5-(3,5-dimethyl-1,2-oxazol-4-yl)-1-[2-(morpholin-4-yl)ethyl]-2-[2-(4-propoxyphenyl)ethyl]-1H-benzimidazole | C29 H36 N4 O3 | 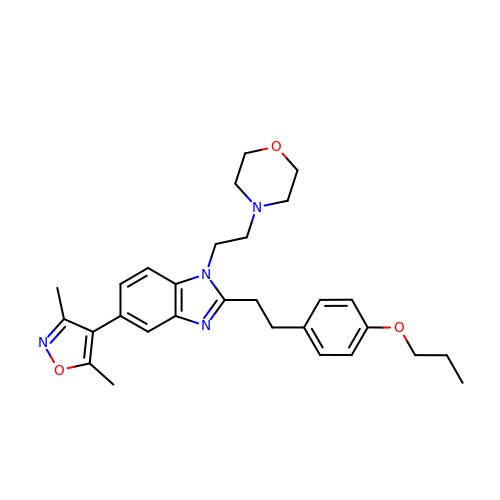CGWBJJZOKGZCSJ-UHFFFAOYSA-N(2S)-2-AMINO-4-(METHYLSULFANYL)-1-(1,3-THIAZOL-2-YL)BUTANE-1,1-DIOL 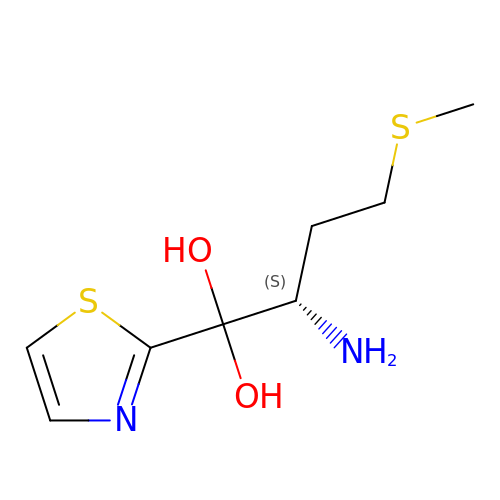| C8 H14 N2 O2 S2 | NPPGNJAWTLSRQG-LURJTMIESA-N>[4x]MGSSHHHHHHMFRTILVANRGEIALRVMRACRELGLRCVAVYSEADRDAPHVAYADDAFLIGPPSPAESYLNIDAIIRAAKATGAEAIHPGYGFLAENASFVRAVTAAGLIFIGPPAEAMERMGGKTAARREATAAGVPVVPGVLEPVTDAAEVRRLGKEFGYPIAIKAVGGGGGRGLRVVRSPEEVDEAFAAARREAEVAFKNGELYVEKYLDDPRHIEIQVLADRYGNAVALGERDCSVQRRHQKLIEECPSPALTPELRAEMGAAAVRLAKAVGYVSAGTLEFLFQDGRYYFLEMNTRIQVEHTVTEMVYGIDLVAAQIRIAQGEKLWFKQEDVVPRGHAIECRINAEDPLHNFRPALGTIGEYHEPVGFGVRVDSGVRAYYTVPSHYDSLLAKLITWGSDRQEAIARMRRALAEYRIEGVTTIIPFHQAALEHPVFTAGAATVNFIPRHPELFSRAAELTPPTAA;>SAGAEPAPEPRRFTIEVNGRRFGVAVFGDGMNATPVASPSRSAPARRAAPKKTTLAAPVDAVISPIQGRVVAVRVAHGQQVEAGQVLFIVEAMKMENEITAPHSGTIAEVRVEVGTTVEAGAMLATYQNTANNTNGK[4x]

Acetyl-CoA carboxylases (ACCs) convert acetyl-CoA to malonyl-CoA, a key step in fatty acid biosynthesis and autotrophic carbon fixation pathways. Three functionally distinct components, biotin carboxylase (BC), biotin carboxyl carrier protein (BCCP), and carboxyltransferase (CT), are either separated or partially fused in different combinations, forming heteromeric ACCs. Here, we identify two BC isoforms (BC1 and BC2) from Chloroflexus aurantiacus, a filamentous anoxygenic phototroph that employs 3-hydroxypropionate (3-HP) bi-cycle rather than Calvin cycle for autotrophic carbon fixation. To investigate the structural basis of BC1 as a bi-functional enzyme, we determined the crystal structures of BC1 and BC2 at 3.2 Å and 3.0 Å resolutions, respectively.

Here, we identify a previously unrecognized C. aurantiacus BC1 that possesses fused BC and BCCP domains, enabling it to exhibit both biotin carboxylase and biotin carrier activities. Crystal structures of BC1 and BC2 at 3.2 Å and 3.0 Å resolutions, respectively, have revealed a BC1 tetramer consisting of two BC1-BC homodimers connected by an eight-stranded β-barrel of the BCCP domain. Although we identified a complete BCCP domain (Ala459-Lys596) in C. aurantiacus BC1, the crystal structure only resolved an N-terminal β-hairpin (Pro466-Gly487) that composed of two antiparallel β-strands. In particular, four β-hairpins cross-interlocked to form an eight-stranded β-barrel, which connected two BC1-BC homodimers at the N-terminal sub-domains to constitute a tetramer. The BC/β-barrel interface was mediated by a symmetrically distributed hydrogen bonding network, which was composed of amino acid residues Glu475, Gly478, Arg479, and Arg480 from the β-hairpin, Tyr32, Arg37, Asp47, Leu50 and Ala72 from the N-terminal sub-domain. Each β-hairpin was stabilized by hydrogen bonding interactions between Phe486-Thr473, Glu475-Ala484, and Asn477-Gly482 amino acid pairs. Specifically, truncation of the amino acid residues that constitute the entire BCCP domain (BC1ΔBCCP, Met1-Glu452) or the β-hairpin (BC1ΔBCCPβ-hairpin, Thr473-Gly486) resulted in a dimer of the BC1 mutants. However, the tetramer formation of BC1 was not affected upon deletion of the BCCP core (BC1ΔBCCPCore, Met1-Lys510). These results indicated that the β-hairpin but not the BCCP core mediated the formation of BC1 tetramer. Overall, these results demonstrated that the β-hairpin mediated tetramer formation is necessary for maintaining effective biotin carboxylase activity of BC1. In the modeled BC1-BC active site, bicarbonate was immobilized through hydrogen bonds with the carboxyl oxygen of Glu295 (2.8 Å), which is conserved with Glu296 in E. coli BC that plays a role in stabilizing the bicarbonate during catalysis.P-NITROPHENYLHYDRAZINE | C6 H7 N3 O2 | 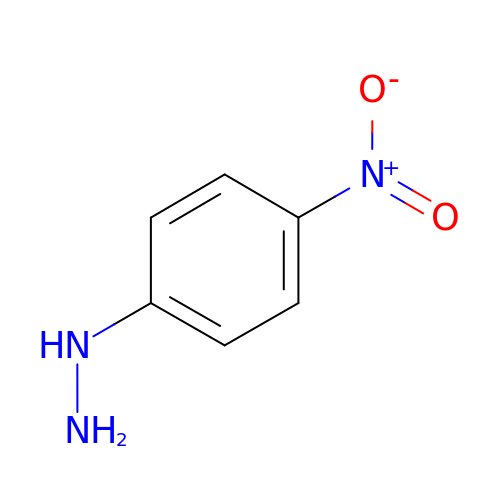KMVPXBDOWDXXEN-UHFFFAOYSA-N>[2x]MGIPAVAEMNPNVNVFVPPRDGFSGPAPRKS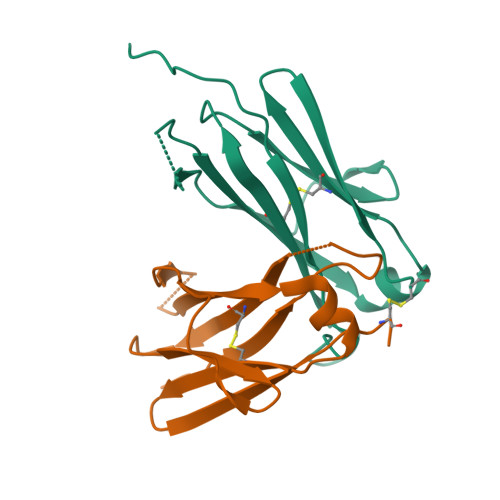KLICEATNFTPKPITVSWLKDGKLVESGFTTDPVTIENKGSTPQTYKVISTLTISEIDWLNLNVYTCRVDHRGLTFLKNVSSTCAA> GPGSSVQLQE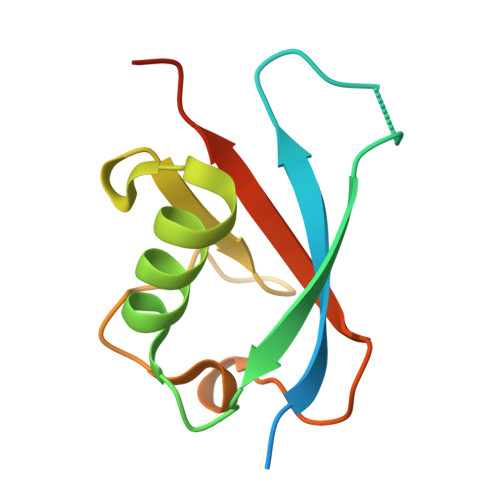ACFPPGPIRLQVTLEDAASAASAASSAHVALQVHPHCTVAALQEQVFSELGFPPAVQRWVIGRCLCVPERSLASYGVRQDGDPAFLYLLSAPREAPAT N-[3-(6-methyl-7-oxo-6,7-dihydro-1H-pyrrolo[2,3-c]pyridin-4-yl)-4-phenoxyphenyl]methanesulfonamide 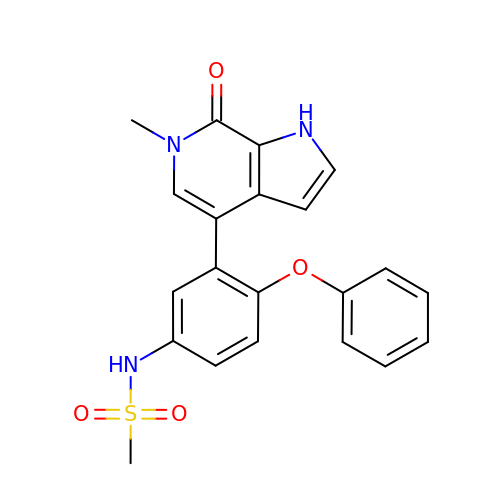| C21 H19 N3 O4 S | JEALBKSAOZOBET-UHFFFAOYSA-N>MTATNKQVILKDYVSGFPTESDFDFTTTTVELRVPEGTNSVLVKNLYLSCDPYMRIRMGKPDPSTAALAQAYTPGQPIQGYGVSRIIESGHPDYKKGDLLWGIVAWEEYSVITPMTHAHFKIQHTDVPLSYYTGLLGMPGMTAYAGFYEVCSPKEGETVYVSAASGAVGQLVGQLAKMMGCYVVGSAGSKEKVDLLKTKFGFDDAFNYKEESDLTAALKRCFPNGIDIYFENVGGKMLDAVLVNMNMHGRIAVCGMISQYNLENQEGVHNLSNIIYKRNRIQGFVVSDFYDKYSKFLEF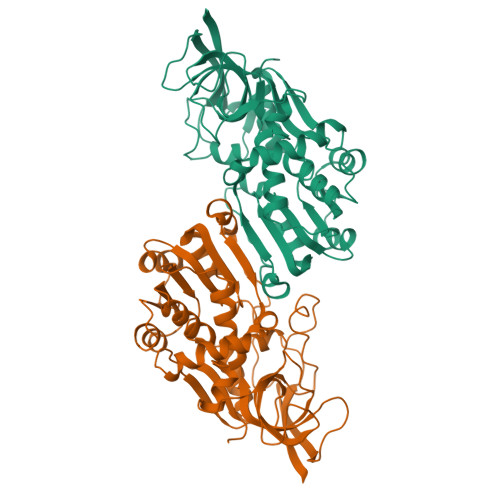VLPHIREGKITYVEDVADGLEKAPEALVGLFHGKNVGKQVVVVARE[2x]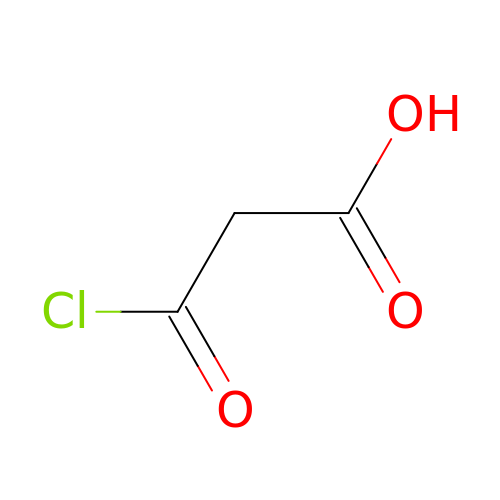3-chloro-3-oxopropanoic acid | C3 H3 Cl O3 | UUOFSRVHZJTWDE-UHFFFAOYSA-N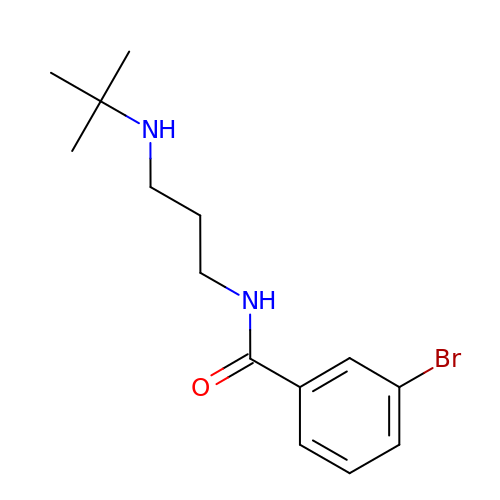3-bromo-N-[3-(tert-butylamino)propyl]benzamide | C14 H21 Br N2 O | XUFUVCIZFNREBI-UHFFFAOYSA-N> N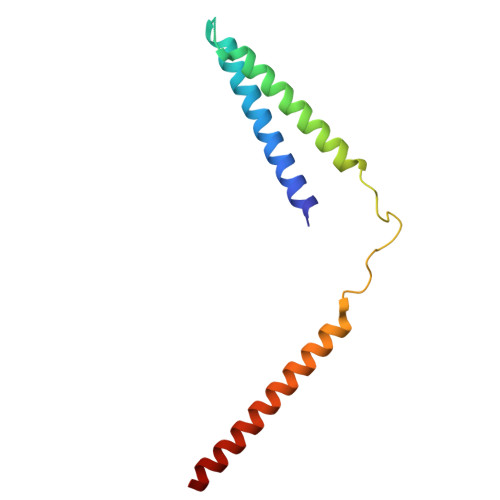ERLRALEDIEREIGAILQNAGTAILELSKEKTNERLLDRQAAAFTTSVQHVEAELSAQIRYLTQVATGQPHEGSSYSSRKDCQMALKRVDYARLKISDVARTCEQML>MGSSHHHHHHSSGLVPRGSHMSNQNAPTPPPTEVIQLDWWKNCVLYQIYPRSFKDSDGDGIGDLKGIISELKHFVDAGVDAIWMSPIFESPMVDFGYDISNFYDIHYEYGTMEDFEELLDKAHELGLKVLLDFVPNHASNESEYFIKSEAREPGYENFFIWADPLPNPENPGVRLPPSNWVSQFGGSAWEWSEKRQQYYLHQFAIQQVDFDFRNPAVKQEMFNIMKFWLDKGADGFRLDALPYLIEADPADHEGRYPDDPLSGLTQFESHQLGYTIPLYTKDLIELYDVVYEWREFLDEYNKNHGGDTRVVFSQGYANVSMTMLYYGNEDGAIGAHFPFNFDFITDLSSKSNARDFV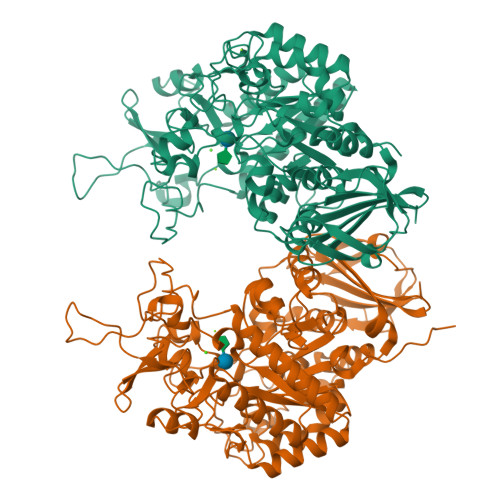YIILRWLTYMPYGGIPNWVFGNHDNNRMPTRFRHDMVDGLNIINMLLPGVAVTYQGEEIGMRDGYVSWEDTVDIEACNRGDPDTYHLYSRDPARTPYHWDNSTSAGFSTSTNTWLPVAEDYQEINLAKQKETARSHFKNYQALTKLRKQATLSHGEYDIRALSDRTFYLVRSLPTHDTYVLLFNVSERRDTVDLGRVPHLTLPATVYVSSIHSARLAGHEITSSQLSLEAGEALVLKAQPI[2x]>[12x]MAHHHHHHMVKIVT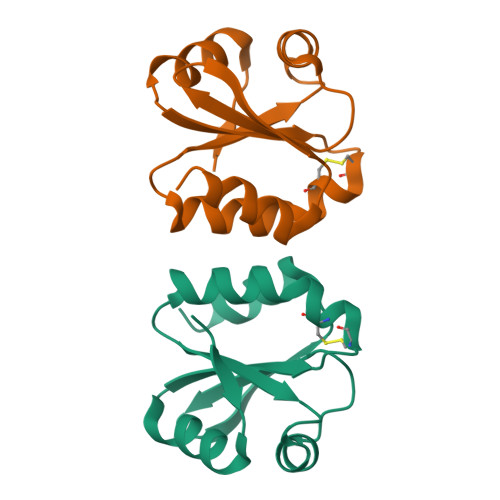SQAEFDSIISQNELVIVDFFAEWCGPCKRIAPFYEECSKTYTKMVFIKVDVDEVSEVTEKENITSMPTFKVYKNGSSVDTLLGANDSALKQLIEKYAA Here, we describe a rhodopsin group found in microorganisms from cold environments, such as glaciers, denoted as CryoRhodopsins (CryoRs). A distinguishing feature of the group is the presence of a buried arginine residue close to the cytoplasmic face. Combining single-particle cryo–electron microscopy and x-ray crystallography with rhodopsin activation by light, we demonstrate that the arginine stabilizes an ultraviolet (UV)–absorbing intermediate of an extremely slow CryoRhodopsin photocycle. Our data suggest that CryoRs are sensors for UV irradiation and are also capable of inward proton translocation modulated by UV light.

For an in-depth investigation, we selected five representatives of the CryoR clade with different seven-letter motifs: RREAEDK (CryoR1, C. levicorallinum, GenBank ID: WP_166787544), RRESEDK (CryoR2, Subtercola sp. AK-R2A1-2, GenBank ID: UFS59673.1), RRETEDK (CryoR3, Cryobacterium frigoriphilum, GenBank ID: WP_166791776), RRDNEDK (CryoR4, Subtercola vilae, UniProt ID: A0A4T2CD69), and RRDTEDK (CryoR5, Subtercola boreus, UniProt ID: A0A3E0VLV3). The transmembrane part is mostly hydrophobic and occupied by lipid molecules as evidenced in the (electron) density maps but has a narrow polar region near the W40 and R43 residues in CryoR1 (Y41 and R44 in CryoR2), which, to some extent, resembles that of the pentameric viral rhodopsin OLPVRII. Next, the cytoplasmic part of the pore in CryoRs has an additional second narrowing formed by the C-terminal residues I238 and E287 in CryoR1 and CryoR2, respectively. In the RSB region of both CryoR1 and CryoR2 up to the arginine residue at the extracellular side (R99/R100 in CryoR1/CryoR2; analog of R82 in BR), there are also no internal water molecules. At the extracellular side of CryoRs, we found a large water-filled cavity, between R99/R100 (in CryoR1/CryoR2; analog of R82 in BR) and the small (single turn) N-terminal α helix, capping the internal space of the CryoR protomer from the extracellular bulk. Our structural data show that in both CryoR1 and CryoR2, the arginine likely plays a triple role. Second, the arginine decreases the pKa of a conserved glutamic acid at the cytoplasmic side (E113/E114 in CryoR1/CryoR2). In that case, R58 (analog of R57 in CryoR1) forms a salt bridge with E114 (analog of E113 in CryoR1) in the ground and M2 states of CryoR2 in almost identical manner to those shown for CryoR1. Thus, structural data on CryoR1 and CryoR2 allow us to conclude that the reorientation of the characteristic unique arginine at the cytoplasmic side of CryoRs in the long-living blue-shifted state is likely a feature of the entire clade.

>[5x]MRLTNVSVPWGATLSNAEHQLIFYFLVVAALAFVAGFIRTYITRNEVGSRYRTAVSARLGMLGVALLAYILIIVAFLLGYDSTAGGWVPNDGAINIFSTRYIEWTVSVPLLTIELLAVCATLGVQARRNTAIAVTATGAMIFCGFLGAIVIDNGTNTGAFILWAVISCVFWVIANVVLIRAVRQSLPTLTPESHTMLKSAAIVLLAGWVVYPIVYFLPLFGASGGLTTTILITLTVADVIVKLGFSTQTHRVAKLRTAEDVRAGDDVHPESIWISSVKQSDAGLPREVYLAEGAAVHDRRTKPPTSAAVASPEAPLPPDSTPLDGGY> RLYRADSRPPDEIKRSGGLMPRGHNEYFDRGTQMNINLYDHARGTQTGFVRYDDGYVSTSLSLRSAHLAGQSILSGYSTYYIYVIATAPNMFNVNDVLGVYSPHPYEQEVSALGGIPYSQIYGWYRVNFGVIDERLHRNREYRDRYYRNLNIAPAEDGYRLAGFPPDHQAWREEPWIHHAPQGCG;> RTITGDTCNEETQNLSTIYLREYQSKVKRQIFSDYQSEVDIYNRI;>[5x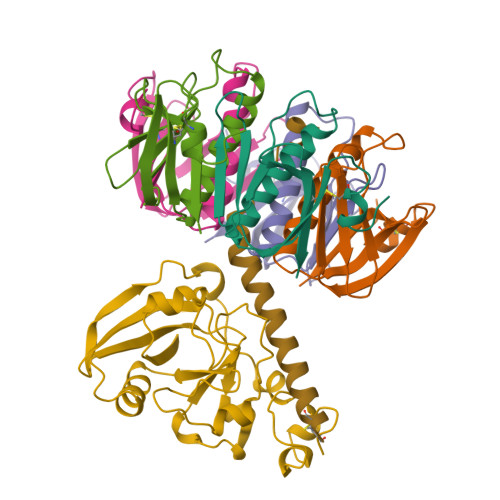]APQTITELCSEYRNTQIYTINDKILSYTESMAGKREMVIITFKSGETFQVEVPGSQHIDSQKKAIERMKDTLRITYLTETKIDKLCVWNNKTPNSIAAISMKN> ANPLYQKHIISINDLSRDDLNLVLATAAKLKANPQPELLKHKVIASCFFEASTRTRLSFETSMHRLGASVVGFSDSANTSLGKKGETLADTISVISTYVDAIVMRHPQEGAARLATEFSGNVPVLNAGDGSNQHPTQTL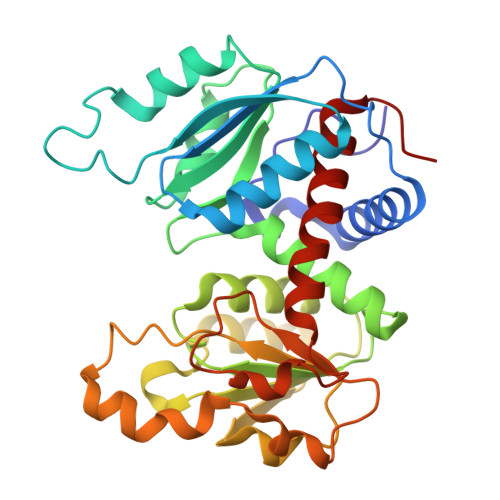LDLFTIQETQGRLDNLHVAMVGDLKYGRTVHSLTQALAKFDGNRFYFIAPDALAMPQYILDMLDEKGIAWSLHSSIEEVMAEVDILYMTRVQKERLDPSEYANVKAQFVLRASDLHNAKANMKVLHPLPRVDEIATDVDKTPHAWYFQQAGNGIFARQALLALVLNRDLVL> HMMENINIVIKDVGYFQDKPQFLNSKSVRQWKHGTKVKLTKHNSHWYTGVVKDGNKSVRGYIYHSMAKVTSKNSDGSVNATINAHAFCWDNKKLNGGDFINLKRGFKGITHPASDGFYPLYFASRKKTFYIPRYMFDIKG;>MMENINIVIKDVGYFQDKPQFLNSKSVRQWKHGTKVKLTKHNSHWYTGVVKDGNKSVRGYIYHSMAKVTSKNSDGSVNATINAHAFCWDNKKLNGGDFINLKRGFKGITHPASDGFYPLYFASRKKTFYIPRYMFDIKK[9x];>HMMENINIVIKDVGYFQDKPQFLNSKSVRQWKHGTKVKLTKHNSHWYTGVVKDGNKSVRGYIY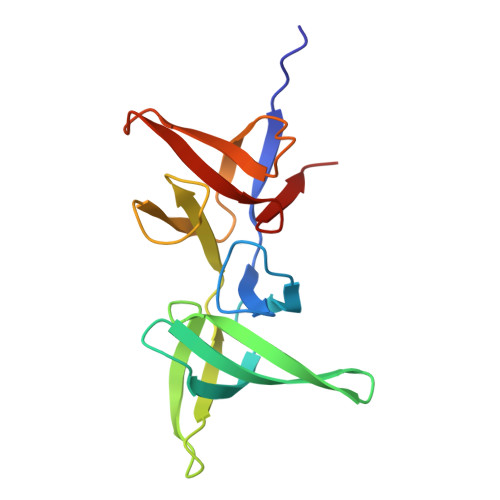HSMAKVTSKNSDGSVNATINAHAFCWDNKKLNGGDFINLKRGFKGITHPASDGFYPLYFASRKKTFYIPRYMFDIKK[2x]> SGNNFEYTLEASKSLRQKPGDSTMTYLNKGQFYPITLKEVSSSEGIHHPISKVRSVIMVVFAEDKSREDQLRHWK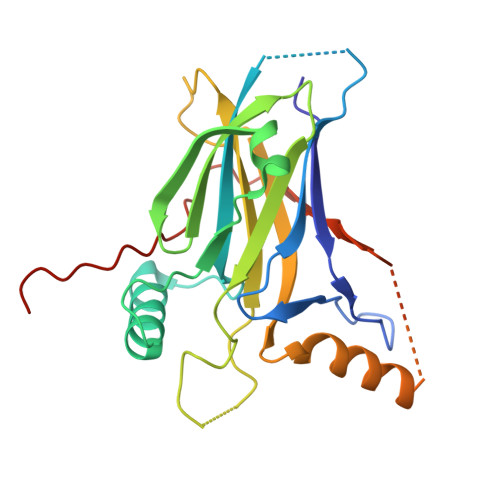YWHSRQHTAKQRCIDIADYKESFNTISNVEEIAYNAISFTWDINDEAKVFISVNCLSTDFSSQKGVKGLPLNIQIDTYSYNNRSNKPVHRAYCQIKVFCDKGAEQKIRDEERKQSKRKVSDVKVPLLPSHKRMDITVFKPFIDLDTQPVLFIPDVHFANLQRG> AKGNDSKDFNNSYGISHITRDNMVKIPQQQNSDQFKVPAFDESTIKNIASAKGKNASGNTIDLDVWDSWPLQNADGTVATYHGYQIVFALAGDPKDSNDTSVYLFYKKAGDKSIDSWKNAGRVFKDSDKFVPNDPHLKNQTQEWSGSGTLTKDGKVRLFYTDYSGKQYGKQTLTTAQVNMSQPNDNTLKVDGVEDYKSIFDGDGKIYQTVQQFIDEGGYDTGDNHTLRAPHYIEDNGHKYLVFEANTGTEDGYQGEDSLYNRAYYGGNNPFFQSEKKKLLEGSNKEKASLANGALGIIELNDDYTLKKVMKPLITSNTVTDEIERANIFKKDGKWYLFTDSRGSKMTIDGIGQDDVYMLGYVSNTLTGKYKPLNDTGLVLHMDLDPNDKTFTYSHFAVPQTKGDNVVITSYM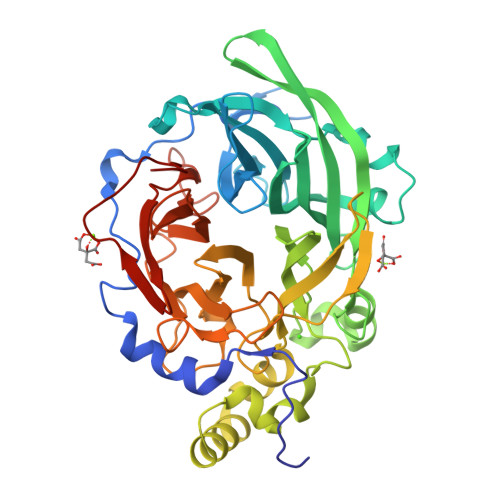TNRGFYEDNHSTFAPSFLVNIDGSKTSVVKDRVLEQGQLTVDED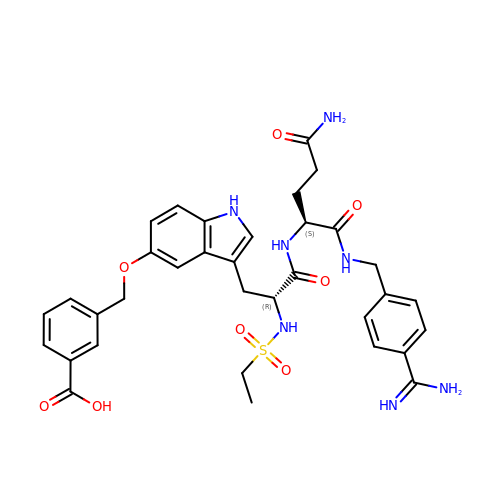3-[[3-[(2R)-3-[[(2S)-5-amino-1-[(4-carbamimidoylphenyl)methylamino]-1,5-dioxo-pentan-2-yl]amino]-2-(ethylsulfonylamino)-3-oxo-propyl]-1H-indol-5-yl]oxymethyl]benzoic acid | C34 H39 N7 O8 S | UDNWHSWDIIAZDA-URLMMPGGSA-N>[12x]SFFSFLGEAFDGARDMWRAYSDMREANYIGSDKYFHARGNYDAAKRGPGGVWAAEAISDARENIQRFF

Systemic AA amyloidosis is a debilitating protein misfolding disease in humans and animals. Serum amyloid A1 (SAA1) is the precursor protein of AA amyloid fibrils. It is an acute phase protein that becomes strongly upregulated during inflammation. Two variants of systemic AA amyloidosis have been described in humans.

In this research, we determined the cryo-EM structures of amyloid fibrils that were isolated from the kidneys of two patients with the vascular variant of systemic AA amyloidosis. Reconstruction of three-dimensional (3D) maps of this fibril morphology achieved, based on the 0.143 Fourier shell correlation (FSC) criterion, a spatial resolution of 2.56 Å for the fibrils from the patient I and of 2.68 Å for the fibrils from patient II. The two 3D maps were highly similar, C1-symmetrical and consisted of two non-equal protein stacks (stacks A and B). Stack A is formed by residues Ser2 to Gly40, while stack B contains residues Ser2 to Phe69, reminiscent of the two groups of fibrils protein obtained by mass spectrometry. The fibril proteins in both stacks show folds that are dominated by β-sheet structure and lack the α-helical conformation of natively folded SAA1. There are four cross-β sheets (β1-β4) in stack A and eight (β1-β8) in stack B. The β-sheets show a notable left-hand twist, which is defined here in the direction of the fibril axis. In the vascular fibril, the Cα atom of Ser2 is 3 Å lower than the Cα atom of Tyr29 in chain A and 5 Å lower in chain B. In the glomerular fibril, the Cα atom of Ser2 is 6 Å higher along the z-axis than the Cα atom of Tyr29. These very different z-axial positions of the N-terminal ends of the fibril proteins lead to the different tilt of the sheet β1 relative to the fibril z-axis, which explains the different directions of the fibril twist of the glomerular and the vascular fibril. While the glomerular fibril shows a symmetrical distribution of the positive and negative charges in the fibril cross-section, the vascular fibril presents a clearly asymmetrical charge distribution. The current vascular structure allows similar conclusions as the fibril protein N-terminus is also buried in the fibril core, indicating that the first has to be removed in order to allow the formation of the fibril structure in the vascular disease variant.> MHPAGIILTKVGYYTIPSMDDLAKITNEKGECIVSDF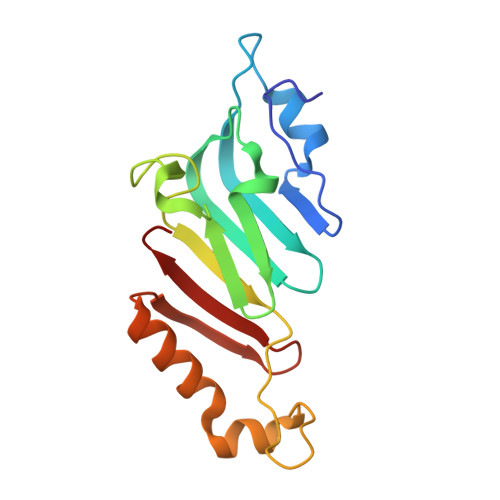TIGRKGYGSIYFEGDVNLTNLNLDDIVHIRRKEVVVYLDDNQKPPVGEGLNRKAEVTLDGVWPTDKTSRCLIKSPDRLADINYEGRLEAVSRKQGAQFKEYRPETGSWVFKVSHF>[3x]GGKKKVCYYYDGDIGNYYYGQGHPMKPHRIRMTHNLLLNYGLYRKMEIYRPHKATAEEMTKYHSDEYIKFLRSIRPDNMSEYSKQMQRFNVGEDCPVFDGLFEFCQLSTGGSVAGAVKLNRQQTDMAVNWAGGLHHAKKSEAS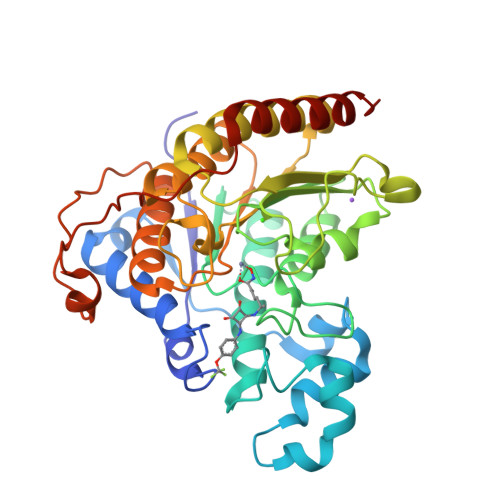GFCYVNDIVLAILELLKYHQRVLYIDIDIHHGDGVEEAFYTTDRVMTVSFHKYGEYFPGTGDLRDIGAGKGKYYAVNFPMRDGIDDESYGQIFKPIISKVMEMYQPSAVVLQCGADSLSGDRLGCFNLTVKGHAKCVEVVKTFNLPLLMLGGGGYTIRNVARCWTYETAVALDCEIPNELPYNDYFEYFGPDFKLHISPSNMTNQNTPEYMEKIKQRLFENLRMLPH>[2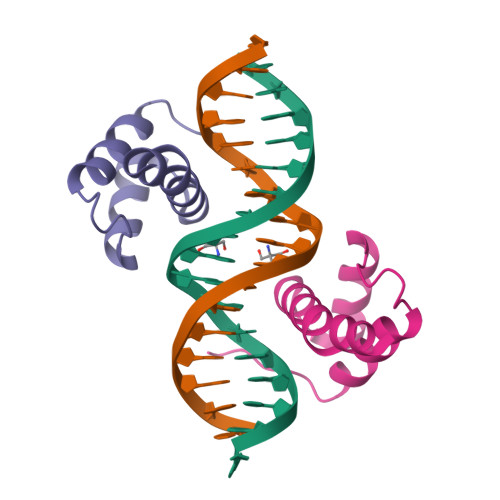x]SMGIFPKVATNIMRAWLFQHLTHPYPSEEQKKQLAQDTGLTILQVNNWFINARRRIVQPMIDQS> GSHMTVFDPTSFTADLLSFMGLNRMESPGHNS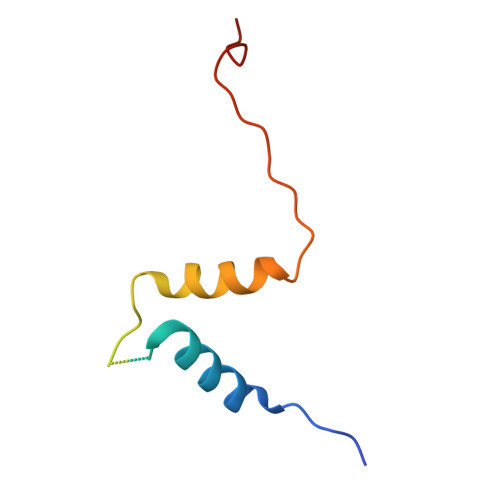ANESDDEGYAGGYLPTDAWQKLGSEAENYFKRTPTFHFMLGSFKTEP Aldehyde dehydrogenases (ALDHs1) are NAD(P)(H)-dependent enzymes found in prokaryotes and eukaryotes that convert a range of aldehyde substrates into their corresponding carboxylic acids. AldA from PtoDC3000 was determined to function as an indole-3-acetaldehyde dehydrogenase through comprehensive metabolic, biochemical, structural, and in planta analyses. AldA was shown to be essential for synthesis of the phytohormone IAA and as a factor contributing to the virulence of PtoDC3000. As with other ALDHs, AldA retains the invariant active site cysteine (Cys302) required for formation of a thioacyl-enzyme intermediate in the reaction sequence and a conserved glutamate (Glu267) that serves to activate a water molecule for hydrolysis of the intermediate.

Enzyme assays using the AldA C302A, E267Q, and E267A mutants showed no detectable activity above background rates in assays using up to 1000-fold higher amounts of protein compared with wild-type AldA. To further examine the reaction mechanism of AldA, the AldA C302A mutant was crystallized in the presence of NAD+ and IAA. The 2.85 Å resolution X-ray crystal structure of the AldA C302A mutant in complex with these ligands was solved by molecular replacement. The overall three-dimensional structure of the AldA C302A mutant is a tetramer with each monomer consisting of an N-terminal NAD(H) binding domain defined by a canonical Rossmann-fold, an interdomain linker, a β-strand oligomerization region, and a C-terminal mixed α/β-domain that includes the catalytic cysteine and the aldehyde substrate binding site. The AldA C302A mutant structure is similar to that of the previously reported wild-type protein with a 0.24 Å2 r.m.s.d. for 497 Cα-atoms in the monomer. NAD+ was observed bound in the N-terminal NAD(H) binding site and IAA in the C-terminal substrate binding site. In the AldA C302A mutant structure, the adenine half of the NAD+ molecule is bound in the same orientation as previously reported for the wild-type enzyme. The nicotinamide half of the coenzyme is bound with the ribose oriented toward Gln349 and the nicotinamide ring pulled away from the catalytic site (defined by the C302A mutation) by contraction of the coenzyme structure. This orientation of NAD+ retains a hydrogen bond between the ligand amide group and the carboxylate side-chain of Glu267, which is positioned into the AldA active site. The IAA carboxylate group is oriented into the catalytic site (i.e., ∼3Å from side-chain of C302A in AldA) with the indole ring positioned by van der Waals interactions in a largely apolar binding site, which includes Gly123, Phe169, Met172, Met173, Trp176, Phe296, Val301, Thr303, Asp459, and Gly461.

>MTTLTRADWEQRAQNLKIEGRAFIQGEYTAAASGETFDCISPVDGRLLAKVASCDAADAQRAVESARSAFDSGAWSRLAPAKRKATMIRFAGLLEQNAEELALLETLDMGKPISDSLGVDIPGGARALSWSGEAIDKLYDEVAATPHDQLGLVTREPVGVVAAIVPWNFPLMMACWKLGPALSTGNSVVLKPSEKSPLTAIRIAQLAIEAGIPAGVLNVLPGYGHTVGKALALHMDVDTVVFTGSTKIAKQLMIYAGESNMKRVWLEAGGKSPNIVFADAPDLQAAADSAASAIAFNQGEVATAGSRLLVERSIKDRFLPMVIEALGTWKPGNPLDPATNVGALVDTQQMNTVLSYIAAGHTDGARLVAGGKQILQETGGTYVEPTIFDGVNNAMRIAQEEIFGPVLSVLTFDTAEEAIQIANDTPYGLAAAVWTANLSKAHLTARALRAGSVWVNQYDGGDMTAPFGGFKQSGNGRDKSLHAFDKYTELKSTWIKL[8x]> HGSSHHHHHHSSGLVPRGSHMASMMAALDSLSLFTSLGLSEQKARETLKNSALSAQLREAATQAQQTLGSTIDKATGILLYGLASRLRDTRRLSFLVSYIASKKIHTEPQLSAALEYVRSHPLDPIDTVDFERECGVGVIVTPEQIEEAVEAAINRHRPQLLVERYHFNMGLLMGEARAVLKWADGKMIKNEVDMQVLHLLGPKLEADLEKKFKVAKARLEETDRRTAKDVVENGETADQTLSLMEQLRGEALKFHKPGENYKTPGYVVTPHTMNLLKQHLEITGGQVRTRFPPEPNGILHIGHAKAINFNFGYAKANNGICFLRFDDTNPEKEEAKFFTAICDM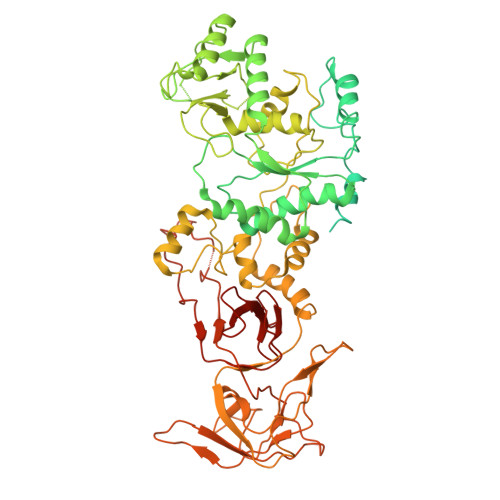VAWLGYTPYKVTYASDYFDQLYAWAVELIRRGLAYVCHQRGEELKGHNTLPSPWRDRPMEESLLLFEAMRKGKFSEGEATLRMKLVMEDGKMDPVAYRVKYTPHHRTGDKWCIYPTYDYTHCLCDSIEHITHSLCTKEFQARRSSYFWLCNALDVYCPVQWEYGRLNLHYAVVSKRKILQLVATGAVRDWDDPRLFTLTALRRRGFPPEAINNFCARVGVTVAQTTMEPHLLEACVRDVLNDTAPRAMAVLESLRVIITNFPAAKSLDIQVPNFPADETKGFHQVPFAPIVFIERTDFKEEPEPGFKRLAWGQPVGLRHTGYVIELQHVVKGPSGCVESLEVTCRRADAGEKPKAFIHWVSQPLMCEVRLYERLFQHKNPEDPTEVPGGFLSDLNLASLHVVDAALVDCSVALAKPFDKFQFERLGYFSVDPDSHQGKLVFNRTVTLKEDPGKV>[2x]MKFAEHLSAHITPEWRKQYIQYEAFKDMLYSAQDQAPSVEVTDEDTVKRYFAKFEEKFFQTCEKELAKINTFYSEKLAEAQRRFATLQNELQSSLDAQKESTGVTTLRQRRKPVFHLSHEERVQHRNIKDLKLAFSEFYLSLILLQNYQNLNFTGFRKILKKHDKILETSRGADWRVAHVEVAPFYTCKKINQLISETEAVVTNELEDGDRQKAMKRLRVPPLGAAQPAPAWTTFRVGLFCGIFIVLNITLVLAAVFKLETDRSIWPLIRIYRGGFLLIEFLFLLGINTYGWRQAGVNHVLIFELNPRSNLSHQHLFE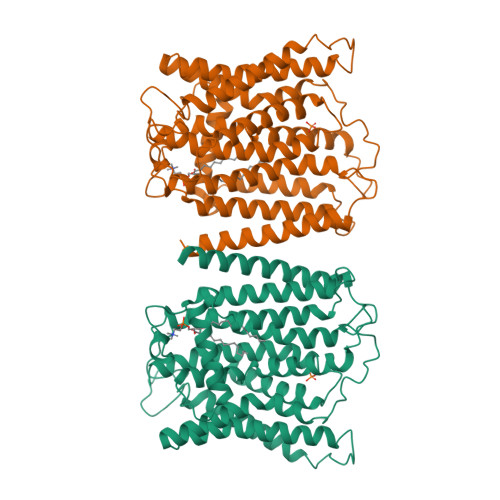IAGFLGILWCLSLLACFFAPISVIPTYVYPLALYGFMVFFLINPTKTFYYKSRFWLLKLLFRVFTAPFHKVGFADFWLADQLNSLSVILMDLEYMICFYSLELKWDESKGLLPNNSEESGICHKYTYGVRAIVQCIPAWLRFIQCLRRYRDTKRAFPHLVNAGKYSTTFFMVTFAALYSTHKERGHSDTMVFFYLWIVFYIISSCYTLIWDLKMDWGLFDKNAGENTFLREEIVYPQKAYYYCAIIEDVILRFAWTIQISITSTTLLPHSGDIIATVFAPLEVFRRFVWNFFRLENEHLNNCGEFRAVRDISVAPLNADDQTLLEQMMDQDDGVRNRQKNRSWKYNQSISLRRPRLASQSKARDTKVLIEDTDDEANTASDYKDDDDK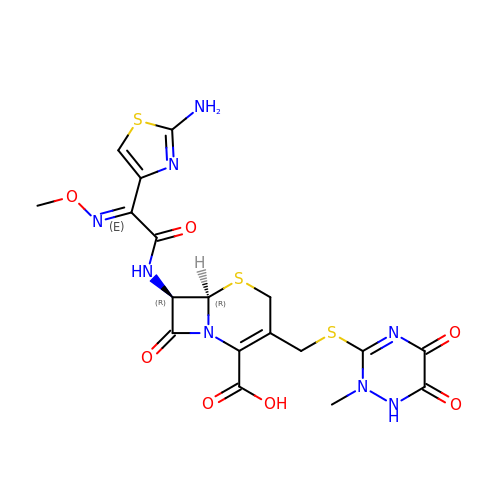Ceftriaxone | C18 H18 N8 O7 S3 | VAAUVRVFOQPIGI-TYHRLYECSA-N> MIVKTEEELQALKEIGYICAKVRNTMQAATKPGITTKELDNIAKELFEEYGAISAPIHDENFPGQTCI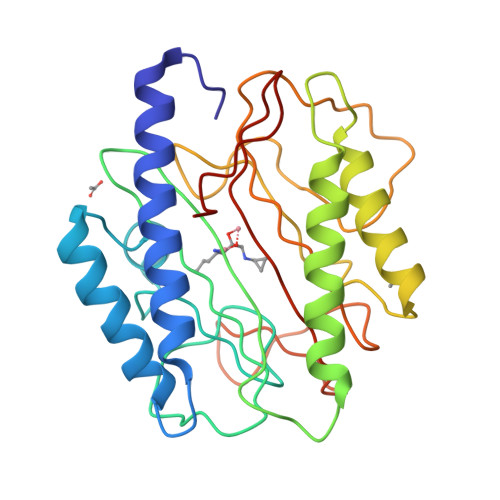SVNEEVAHGIPSKRVIREGDLVNIDVSALKNGYYADTGISFVVGESDDPMKQKVCDVATMAFENAIAKVKPGTKLSNIGKAVHNTARQNDLKVIKNLTGHGVGLSLHEAPAHVLNYFDPKDKTLLTEGMVLAIEPFISSNASFVTEGKNEWAFETSDKSFVAQIEHTVIVTKDGPILTTKIEEE>MGSSHHHHHHSSGRENLYFQGMPSLTPRCIIVRHGQTEWSKSGQYTGLTDLPLTPYGEGQMLRTGESVFRNNQFLNPDNITYIFTSPRLRARQTVDLVLKPLSDEQRAKIRVVVDDDLREWEYGDYEGMLTREIIELRKSRGLDKERPWNIWRDGCENGETTQQIGLRLSRAIARIQNLHRKHQSEGRASDIMVFAHGHALRYFAAIWFGLGVQKKCETIEEIQNVKSYDDDTVPYVKLESYRHLVDNPCFLLDAGGIGVLSYAHHNIDEPALELAGPFVSPPEEESQHGD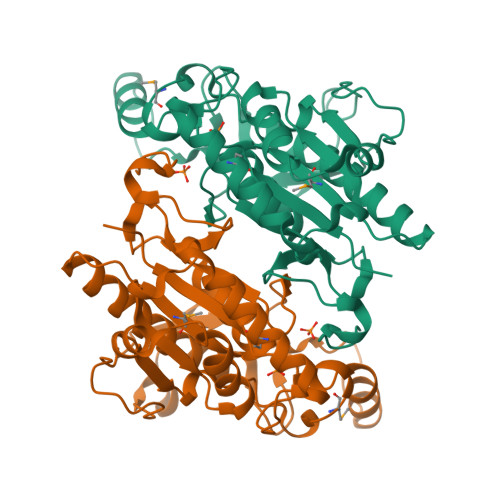V[4x]> LNMSGIALSRLAQERKAWRKDHPFGFVAVPTKNPDGTMNLMNWECAIPGKKGTPWEGGLFKLRMLFKDDYPSSPPKCKFEPPLFHPNVYPSGTVCLS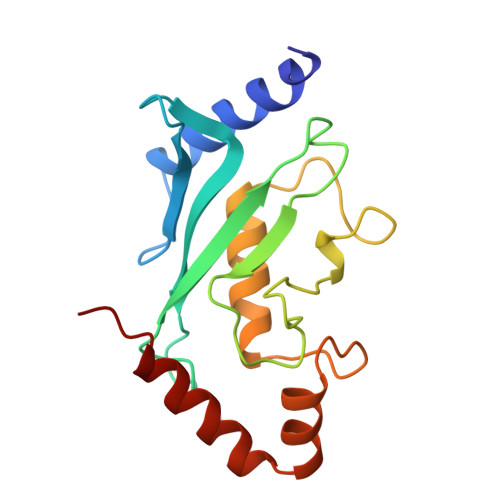ILEEDKDWRPAITIKQILLGIQELLNEPNIQDPAQAEAYTIYCQNRVEYEKRVRAQAKKFAPS>MAESRSPDRGAKEDKPRPRNISREESLQLEGYKHACHALLHAPSQAKLFDRVPIRRVLLMMMRFDGRLGFPGGFVDTRDISLEEGLKRELEEELGPALATVEVTEDDYRSSQVREHPQKCVTHFYIKELKLEEIERIEAEAVNAKDHG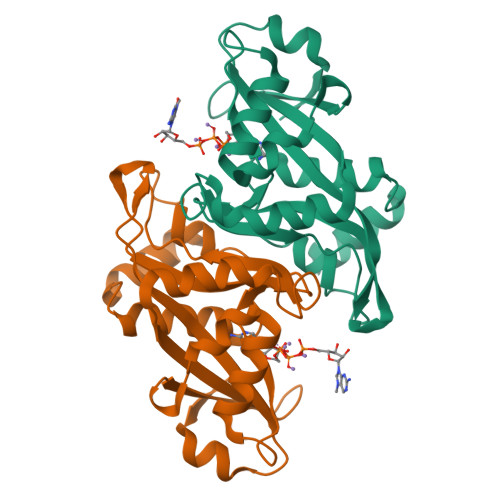LEVMGLIRVPLYTLRDRVGGLPAFLCNNFIGNSKSQLLYALRSLKLLREDQIQEVLKASHRLQY[2x]S. pneumoniae produces up to three distinct sialidase enzymes: NanA, NanB, and NanC. NanC is an unusual sialidase in that its primary reaction product is 2-deoxy-2,3-didehydro-N-acetylneuraminic acid (Neu5Ac2en, also known as DANA), a nonspecific hydrolytic sialidase inhibitor. NanC adopts the same overall topology as seen in NanA and NanB, with a CBM (residues 85–271), followed by a catalytic domain (residues 272–740). The catalytic domain adopts the canonical glycoside hydrolase family 33 sialidase, six-bladed β-propeller fold shared by viral, bacterial, and mammalian sialidases.

Structures of NanC have been determined with Neu5Ac2en, 3F-β-Neu5Ac, and OC bound at the catalytic active site. Thus, many of the Neu5Ac2en to NanC interactions are also conserved with NanA and NanB. These include an arginine triad, comprised of Arg-290, Arg-600, and Arg-662, which orients the ligand in the active site via electrostatic interactions with the Neu5Ac2en carboxylate. The ligand sits on top of the catalytic pair of Glu-584 and Tyr-695 and beneath the general acid base Asp-315. The latter residue is substantially closer to the C2 of Neu5Ac2en than in NanA or NanB Neu5Ac2en complexes: 3.2 Å in comparison with 4.2 and 4.5 Å, respectively (Refs. 23 and 24). The most significant structural change observed upon binding and/or formation of Neu5Ac2en is the substantial shift in Phe-316 and Phe-396 of the hydrophobic pocket and the loop upon which the latter resides (herein named the 396 loop, residues 392–401). The Cα of Phe-396 advances 2.1 Å into the active site, and the side chain changes conformation, moving out of the active site to accommodate the ligand. The net result of the movement of the 396 loop is that it partially constricts the active site. The movement appears to be stabilized by hydrophobic interactions between Phe-396 and the C9 carbon of Neu5Ac2en because no hydrogen bonds or other stabilizing interactions are formed between the residues of the 396 loop and Neu5Ac2en. When short Neu5Ac2en soaks were performed, the CBM binding site was empty, whereas bound Neu5Ac became apparent when the soaking time was increased.

>MAHHHHHHSSGLEVLFQGPNTPVLEKNNVTLTGGGENVTKELKDKFTSGDFTVVIKYNQSSEKGLQALFGISNSKPGQQNSYVDVFLRDNGELGMEARDTSSNKNNLVSRPASVWGKYKQEAVTNTVAVVADSVKKTYSLYANGTKVVEKKVDNFLNIKDIKGIDYYMLGGVKRAGKTAFGFNGTLENIKFFNSALDEETVKKMTTNAVTGHLIYTANDTTGSNYFRIPVLYTFSNGRVFSSIDARYGGTHDFLNKINIATSYSDDNGKTWTKPKLTLAFDDFAPVPLEWPREVGGRDLQISGGATYIDSVIVEKKNKQVLMFADVMPAGVSFREATRKDSGYKQIDGNYYLKLRKQGDTDYNYTIRENGTVYDDRTNRPTEFSVDKNFGIKQNGNYLTVEQYSVSFENNKKTEYRNGTKVHMNIFYKDALFKVVPTNYIAYISSNDHGESWSAPTLLPPIMGLNRNAPYLGPGRGIIESSTGRILIPSYTGKESAFIYSDDNGASWKVKVVPLPSSWSAEAQFVELSPGVIQAYMRTNNGKIAYLTSKDAGTTWSAPEYLKFVSNPSYGTQLSIINYSQLIDGKKAVILSTPNSTNGRKHGQIWIGLINDDNTIDWRYHHDVDYSNYGYSYSTLTELPNHEIGLMFEKFDSWSRNELHMKNVVPYITFKIEDLKKN[2x]>[2x]ALWGPLQDSLEHTLRVAIAHYQDDPDLRFLLDQVQLGLRCCGAASYQDWQQNLYFQCSSPGVQA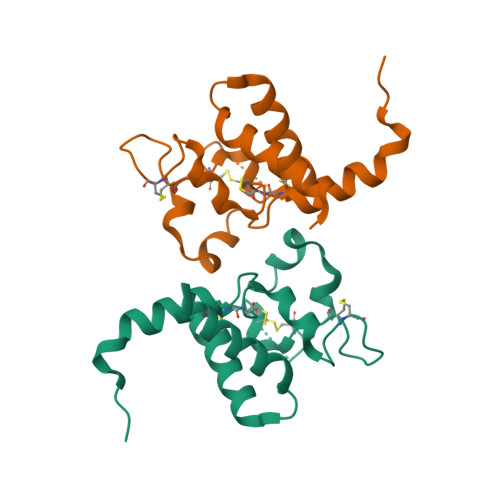CSLPASCCIDPREDGASVNDQCGFGVLRLDADAAQRVVYLEGCGPPLRRWLRANLENLYFQ>[4x]GMEPFKQQKVEDFYDIGEELGSGQFAIVKKCREKSTGLEYAAKFIKKRQSRASRRGVSREEIEREVSILRQVLHHNVITLHDVYENRTDVVLILELVSGGELFDFLAQKESLSEEEATSFIKQILDGVNYLHTKKIAHFDLKPENIMLLDKNIPIPHIKLIDFGLAHEIEDGVEFKNIFGTPEFVAPEIVNYEPLGLEADMWSIGVITYILLSGASPFLGDTKQE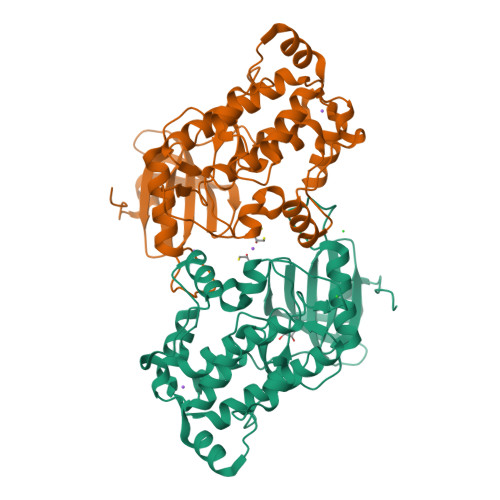TLANITSVSYDFDEEFFSHTSELAKDFIRKLLVKETRKRLTIQEALRHPWITPVDNQQAMVRRESVVNLENFRKQYVRRRWKLSFSIVSLCNHLTR KtrAB is a cation channel with a nucleotide-dependent RCK domain. The structure of the KtrAB complex revealed a homodimeric membrane protein (KtrB) assembled with a cytosolic RCK octameric ring, formed by the KtrA protein. KtrA binds nucleotides, ATP or ADP. ATP binding induces the adoption of a square-conformation by the octameric ring and increased K+ flux activity through KtrAB; ADP binding results in a non-square conformation and decreased flux.

As a control, we also analyzed the impact of mutating A80 since substitution with a bulkier side-chain was expected to cause a distortion of the nucleotide-binding site. As expected, A80P resulted in KtrAB inactivation. To understand the basis of these results we first verified that the KtrA mutants A80P and E125Q retained the same basic properties of the wild-type protein. Both mutants assemble as octamers and are able to form a stable complex with KtrB, as revealed by size-exclusion chromatography. Crystal structures of the mutants that did not rescue the TK2420 growth phenotype (A80P and E125Q) reveal a different picture. The ATP-bound structures do not adopt a square conformation, displaying L1/L2 distances for A80P (at 3.9 Å resolution) of 52/23 Å and for E125Q (at 4.1 Å resolution and with two different half-rings in the asymmetric unit) of 34/30 Å and 42/27 Å. In contrast, mutants that do not rescue growth (A80P and E125Q) also do not adopt the square conformation in the ATP-bound structures. Importantly, this offset was not the result of the refinement procedure since the position of the residue is very similar to the one in the wild-type structure. It is obvious from the maps that adjustment of the main-chain position of the residue into the density would impinge on the ATP molecule, requiring a shift in the nucleotide position to avoid steric-clashes. We concluded therefore that the A80P mutation causes a distortion of the main-chain and leads to an alteration in the position of the ATP, impeding the adoption of the square conformation.

>MGRIKNKQFAVIGLGRFGGSICKELHRMGHEVLAVDINEEKVNAYASYATHAVIANATEENELLSLGIRNFEYVIVAIGPNIQASTLTTLLLKELDIPNIWVKAQNYYHHKVLEKIGADRIIHPEKDMGVKIAQSLSDENVLNYIDLSDEYSIVELLATRKLDSKSIIDLNVRAKYGCTILAIKHHGDICLSPAPEDIIREQDCLVIMGHKKDIKRFENEGM[8x]>[6x]ERTINLYPLTNYTFGTKEPLYEKDSSVAARFQRMREEFDKIGMRRTVEGVLIVHEHRLPHVLLLQLGTTFFKLPGGELNPGEDEVEGLKRLMTEILGRQDGVLQDWVIDDCIGNWWRPNFEPP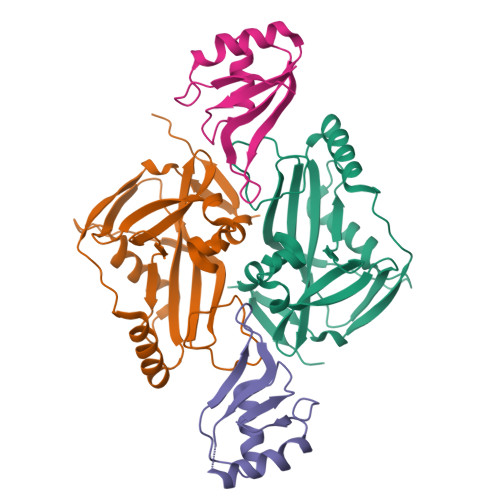QYPYIPAHITKPKEHKKLFLVQLQEKALFAVPKNYKLVAAPLFELYDNAPGYGPIISSLPQLLSRFNFIYNLEHHHHHH;>RIALYIGNLTWWTTDEDLTEAVHSLGVNDILEIKFFENRANGQSKGFALVGVGSEASSKKLMDLLPKRELHGQNPVVTPSNKLEHHHHHH[6x]> DECAIAAQQCT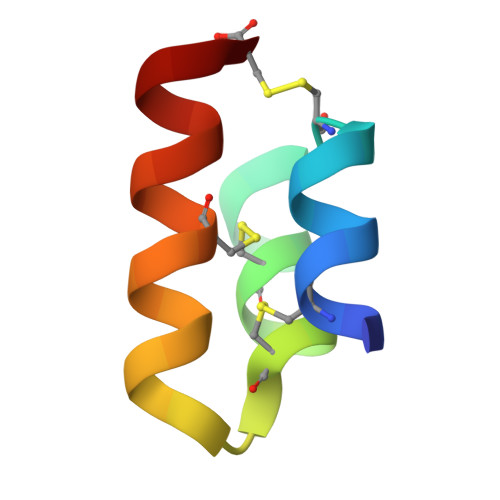NEEGCDAACAPDPEATMGCLMYIWNNC> HTVSPVNPNAQQTTKTVMNWLAHLPNRTENRVLSGAFGGYSHDTFSMAEADRIRSATGQSPAIYGCDYARGWLETANIEDSIDVSCNGDLMSYWKNGGIPQISLHLANPAFQSGHFKTPITNDQYKNILDSATAEGKRLNAMLSKIADGLQELENQGVPVLFRPLHEMNGEWFWWGLTSYNQKDNERISLYKQLYKKIYHYMTDTRGL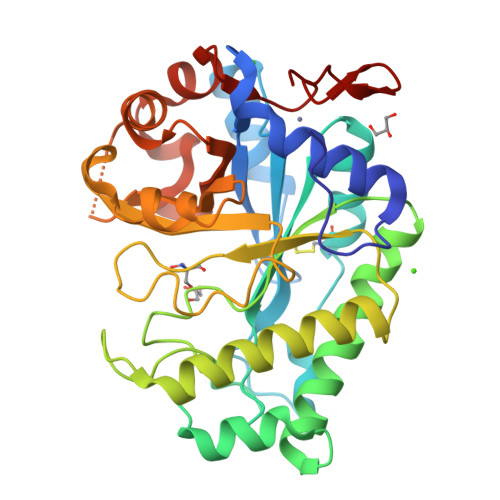DHLIWVYSPDANRDFKTDFYPGASYVDIVGLDAYFQDAYSINGYDQLTALNKPFAFTEVGPQTANGSFDYSLFINAIKQKYPKTIYFLAWNDEWSAAVNKGASALYHDSWTLNKGEIWNGDSLTPIVE> MENPHEQVQANILSRIIGNVKRLNESVAILNQELVTINNRNKNLEIMGAICDNYHSSVQFNLEATN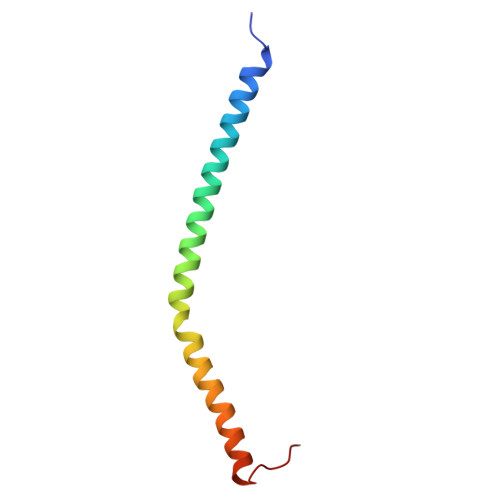NKKPPL> MDTEVSNHNYTQAVAYLNRATSSCVKKCDSLNNNGSLSSKQESCLKTCAE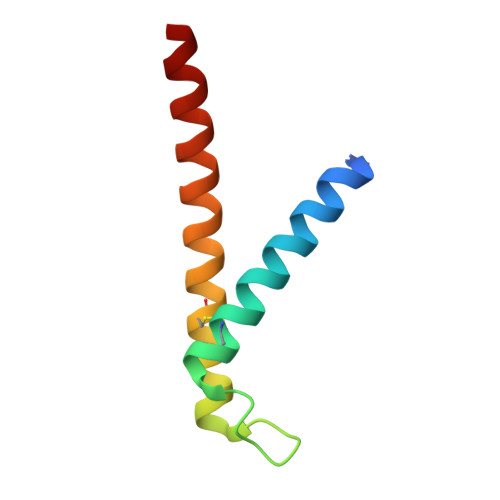NHAIATKIHAEYIRKLAESKYL However, we found that TMEM106B forms amyloid fibrils not only in the diseased brain, but also in the brains of normal elders. Moreover, cryo-EM structure determination of these ex vivo fibrils showed that they share similar structures, in which TMEM106B adopts a curling stone-like fold composed of residues 120–254 that originally form the luminal domain of TMEM106B in its native fold. In the native state, TMEM106B is cleaved by lysosomal proteases, which leads to the formation of the N-terminal fragment and the luminal domain. Thus, the structure of TMEM106B in the fibrillar state indicates that prior to forming amyloid fibrils, the luminal domain is cleaved off at Arg119.

The PDD patient was in the late stage of PD and manifested severe dementia symptom. We then were able to unambiguously fit TMEM106B molecules into the cryo-EM density maps and build structural models for the fibrils from normal 2 (referred to as Type 1) and the major species of PDD (referred to as Type 2). In total, we obtained three types of fibril structures (polymorphs) from four fibril species extracted from the brains of three donors: Type 1 fibril in normal 2, Type 2 in normal 1 and PDD, and Type 3 in PDD. The Type 2 TMEM106B structure fits well in both density maps, except that TMEM106B dimerizes in the minor fibril species of PDD (referred to as Type 3) via electrostatic interactions between R178, K180 and an unknown density. TMEM106B conformations in Type 2 and Type 3 (dimer) are nearly identical, while that in Type 1 is moderately different from the other two. The fibril cores of Type 1 and Type 2 both consist of residues 120–254 of TMEM106B forming 17 β-strands, which are arranged into a curling stone-like fold. Residues 120–160 build the handle of the curling stone and are nearly identical in conformation in both Type 1 and Type 2 fibrils. In contrast to the identical N-terminal handle part of the structure, the stone part of Type 1 and Type 2 exhibits conformational variations. The overall fold of Type 2 is rather flat, while the stone part of Type 1 swaps between neighboring rungs. The protein segment (residues 174–186) forms a hydrophobic hole in Type 2, in which unknown densities were observed in the fibrils from normal 1 and PDD.

>SIDVKYIGVKSAYVSYDVQKRTIYLNITNTLNITNNNYYSVEVENITAQVQFSKTVIGKARLNNITIIGPLDMKQIDYTVPTVIAEEMSYMYDFCTLISIKVHNIVLMMQVTVTTTYFGHSEQISQERYQYVDCG[3x]> MFRTFGRRLVSCTLPLLQSAPHDLPEGFEFMEHKVVNKDIHAPHENLETLRLTLTRQDEFLLREEPVKCV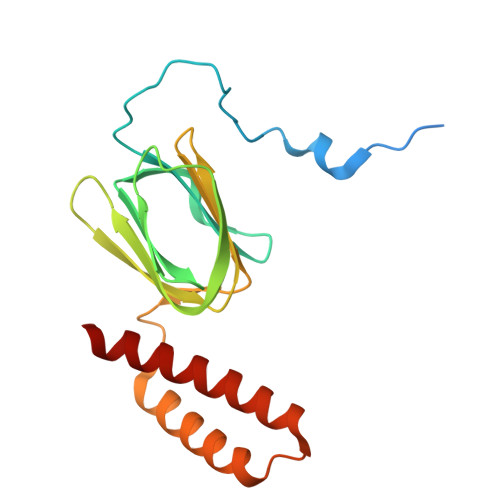TVTGTNGEYGIYPGHAYKIVQLNPSPLTVEYTDGTTKKYFVSGGFAHINNEGSCDVNTVECTLLDDLDLAIAEKELAAQQAALGSAKDDKAKSVVEIRISVIEAVIAALKHH>MNGTVKKMNGARRPHGLASILAIGTANPSNCFNQDEFPDYSFRVTKSEHLTSLKDKFKRICERSTVRKRYLHLTEELLQEYPSIATYDAPSLDARQEIEVAEVPKLAARAASRAIEEWGQPKNKITHLIFSSTSGIEKPGVDCHLVHLLGLPLSVNRVMLYTIGCHAGGTVLRIAKDLAENNVGSRVLVVCSELTVMTFRGPSETDLANLIRMGIFGDGAAALIIGADPDLSIEKPIFEIFSASQTLVPNTSKAIRGRVKEMGLTFYVDKMVPTLVASNIEQCLDKAFSPLGINDWNSIFWIPHPGGPAILAEIEAKLELKPGKLRATRHVLSEYGNMSGATVLFILDEMRRRSKKEGKGTTGDGLEWGVLMGFGPGVTVETIV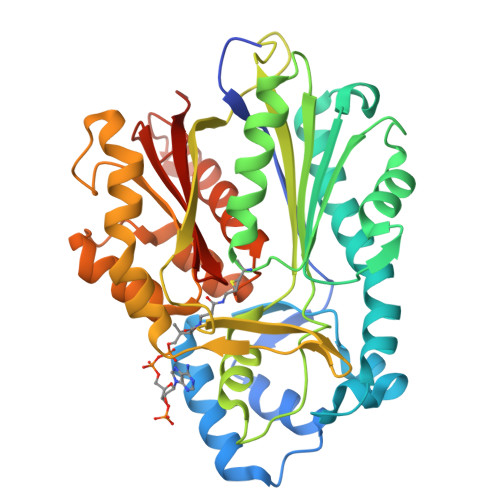LRAISVVTE[8x]>[2x]KPYTIDKANSSVWFEVKHFKFNETRGVFDSFDGKIDADPNTKALNVFEGKIDIKSINTRNKKRDDHLKTAE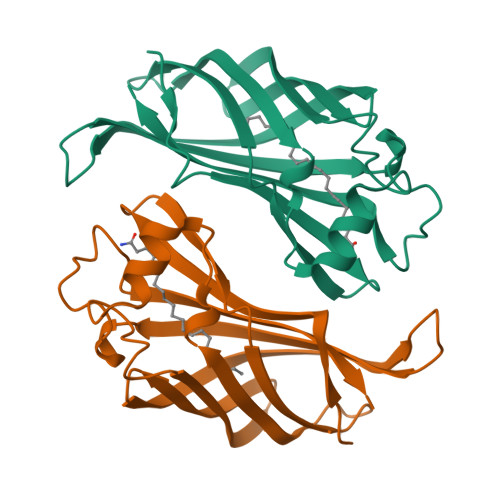FFDVVKYPKGSFKMTKYEDGKIHGDLTLHGVTKPVVLEAKIQAPLQNPMNKKEFMVLQAEGKINRKDFGIGKTFSDAVVGDEVKIELKLEAYA> MKLYYKVGACSLAPHIILSEAGLPYELEAVDLKAKKTADGGDYFAVNPRGAVPALEVKPGTVITQNAAILQYIGDHSD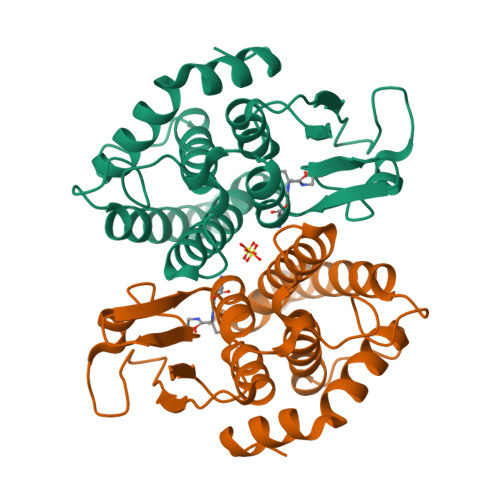VAAFKPAYGSIERARLQEALGFCSDLHAAFSGLFAPNLSEEARAGVIANINRRLGQLEAMLSDKNAYWLGDDFTQPDAYASVIIGWGVGQKLDLSAYPKALKLRERVLARPNVQKAFKEEGLN>[2x]GFGNNVKVEAIINNWAQKDYKLLSADKGITGFSVSNISII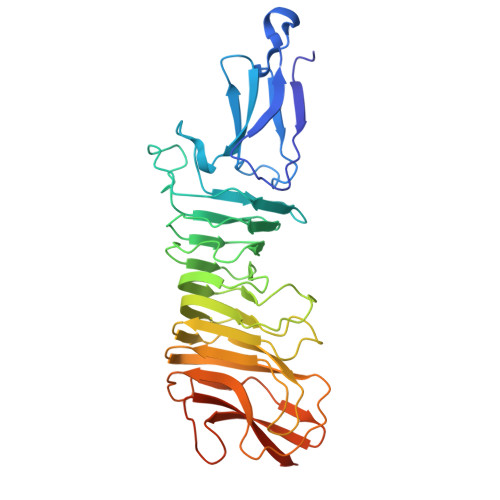NPLLTTGAIDYTKSYISDQNKLIYGLSWNDTDGDSHGEFNLKENAELTVSTILADNLSHHNINSWDGKSLTKSGEGTLILAEKNTYSGFTNINAGILKMGTVEAMTRTAGVIVNKGATLNFSGMNQTVNTLLNSGTVLINNINAPFLPDPVIVTGNMTLEKNGHVILNNSSSNVGQTYVQKGNWHGKGGILSLGAVLGNDNSKTDRLEIAGHASGITYVAVTNEGGSGDKTLEGVQIISTDSSDKNAFIQKGRIVAGSYDYRLKQGTVSGLNTNKWYLTSQMDNQESKQMSNQESTQMSSR> MVSKNKKLNLKDKYQYLTRDMAWEPTYQDKKDIFPEEDFEGIKITDWSQWEDPFRLTMDAYWKYQAEKEKKLYAIFDAFAQNNGHQNISDARYVNALKLFISGISPLEHAAFQGYSKVGRQFSGAGARVACQMQAIDELRHSQTQQHAMSHYNKHFNGLHDGPHMHDRVWYLSVPKSFFDDARSAGPFEFLTAISFSFEYVLTNLLFVPFMSGAAYNGDM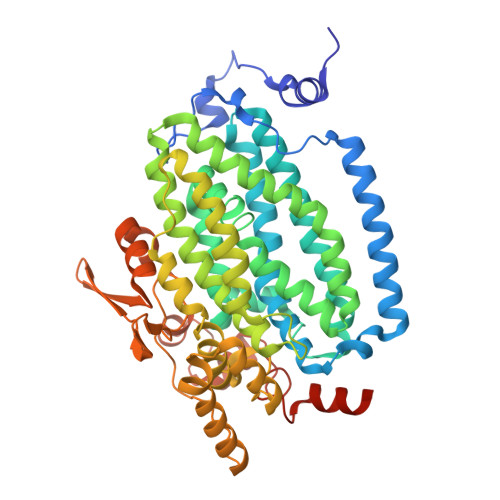ATVTFGFSAQSDEARHMTLGLEVIKFILEQHEDNVPIVQRWIDKWFWRGFRLLSLVSMMMDYMLPNKVMSWSEAWEVYYEQNGGALFKDLERYGIRPPKYQDVANDAKHHLSHQLWTTFYQYCQATNFHTWIPEKEEMDWMSEKYPDTFDKYYRPRYEYLAKEAAAGRRFYNNTLPQLCQVCQIPTIFTEKDAPTMLSHRQIEHEGERYHFCSDGCCDIFKHEPEKYIQAWLPVHQIYQGNCEGGDLETVVQKYYHINIGEDNFDYVGSPDQKHWLSIKGRKPADKNQDAA>[2x]GSFTARPSSSMADFRKFFAKAKHIVIISGAGVSAESGVPTFRGAGGYWRKWQAQDLATPLAFAHNPSRVWEFYHYRREVMGSKEPNAGHRAIAECETRLGKQGRRVVVITQNIDELHRKAGTKNLLEIHGSLFKTRCTS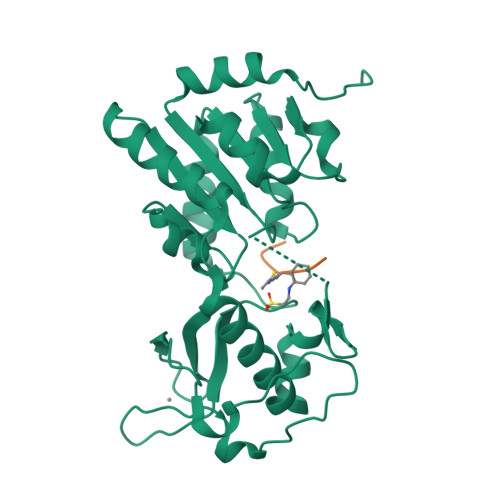CGVVAENYKSPICPALSGKGAPEPGTQDASIPVEKLPRCEEAGCGGLLRPHVVWFGENLDPAILEEVDRELAHCDLCLVVGTSSVVYPAAMFAPQVAARGVPVAEFNTETTPATNRFRFHFQGPCGTTLPEALA;>[2x]KQTARXSTGGKA> GSHMNTAEEDMEDDTSWRSEATFQFTVERFSRLSESVLSPPCFVRNLPWKIMVMPRFYPDRPHQKSVGFFLQCNAESDSTSWSCHAQAVLKIINYRDDEKSFSRRISHLFFHKENDWGFSNFMAWSEVTDPEKGFIDDDKVTFEVFVQADLDAGVSEHS

Herpesvirus-associated ubiquitin-specific protease (HAUSP, also known as USP7), a deubiquitylating enzyme of the ubiquitin-specific processing protease family, specifically deubiquitylates both p53 and MDM2, hence playing an important yet enigmatic role in the p53–MDM2 pathway. Here we demonstrate that both p53 and MDM2 specifically recognize the N-terminal tumor necrosis factor–receptor associated factor (TRAF)–like domain of HAUSP in a mutually exclusive manner. The crystal structures of the HAUSP TRAF-like domain in complex with p53 and MDM2 peptides, determined at 2.3-Å and 1.7-Å resolutions, respectively, reveal that the MDM2 peptide recognizes the same surface groove in HAUSP as that recognized by p53 but mediates more extensive interactions. Structure-based sequence alignment of the three HAUSP-binding peptides revealed a conserved four-residue binding motif with the consensus sequence of (Ø/E)-G-(Ø/G)-S, where Ø denotes a non-polar residue.

After many unsuccessful trials, we once again succeeded by engineering a chimeric protein with the MDM2 peptide (residues 223–232) fused to the C-terminus of the HAUSP TRAF-like domain (residues 53–197). We crystallized this chimeric protein and solved its structure at 1.7-Å resolution. In the structure of the HAUSP–MDM2 fusion protein, the MDM2 peptide (residues 223–230) is bound to the shallow surface groove on one side of the β-sandwich in the TRAF-like domain, the same site where p53 binds. The MDM2 peptide assumes an extended main-chain conformation, extending across strands β3, β4, β6, and β7. Five residues in the MDM2 peptide, Asp225-Ala226-Gly227-Val228-Ser229, make extensive polar and non-polar interactions with the surface-binding residues from all four strands, particularly strand β7. At the N-terminal end of the MDM2 peptide, the carboxylate side chain of Asp225 accepts a charge-stabilized hydrogen bond from the guanidinium group of Arg152 in HAUSP. The side chain of Ala226 in MDM2 packs against a hydrophobic pocket formed by the backbone Cα atom of Gly166 and the side chains of Phe167, Trp165, and Ile154 in HAUSP. The main-chain groups of Gly227 in MDM2 make two hydrogen bonds to Gly166 in HAUSP, whereas the backbone Cα atom of Gly227 is within van der Waals–contact distance of the hydrophobic side chain of Trp165 in HAUSP. At the C-terminal end of the MDM2 peptide, Ser229 in MDM2 makes a total of three hydrogen bonds to surface residues in HAUSP. Compared to p53, the more extensive interactions between MDM2 and HAUSP provide a mechanistic explanation to our biochemical observation that MDM2 out-competed excess p53 for binding to HAUSP.> MAESKPTPQSTFTGPIVVDPITRIEGHLRIMVEVENGKVKDAWSSSQLFRGLEIILKGRDPRDAQHFTQRACGICTYVHALASSRCVDDAVKVSIPANARMMRNLVMASQYLHDHLVHFYHFHALDWVDVTAALKADPNKAAKLAASIAPARPGNSAKALKAVQDKLKAFVESGQLGIFTNAYFLGGHKAYYLPPEVDLIATAHYLEALHMQVKAASAMA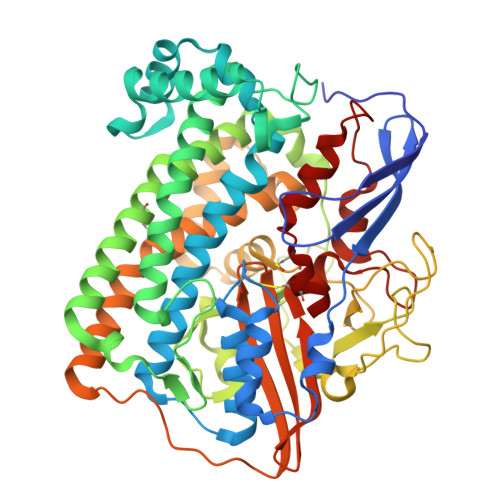ILGGKNPHTQFTVVGGCSNYQGLTKDPLANYLALSKEVCQFVNECYIPDLLAVAGFYKDWGGIGGTSNYLAFGEFATDDSSPEKHLATSQFPSGVITGRDLGKVDNVDLGAIYEDVKYSWYAPGGDGKHPYDGVTDPKYTKLDDKDHYSWMKAPRYKGKAMEVGPLARTFIAYAKGQPDFKKVVDMVLGKLSVPATALHSTLGRTAARGIETAIVCANMEKWIKEMADSGAKDNTLCAKWEMPEESKGVGLADAPRGALSHWIRIKGKKIDNFQLVVPSTWNLGPRGAQGDKSPVEEALIGTPIADPKRPVEILRTVHAFDPCIACGVH>MLGLKTSIIGRRVIYFQEITSTNEFAKTSYLEEGTVIVADKQTMGHGALNRKWESPEGGLWLSIVLSPKVPQKDLPKIVFLGAVGVVETLKEFSIDGRIKWPNDVLVNYKAIAGVLVEGKGDKIVLGIGLNVNNKVPNGATSMKLELGSEVPLLSVFRSLITNLDRLYLNFLKNPMDILNLVRDNMILGVRVKILGDGSFEGIAEDIDDFGRLIIRLDSGEVKKVIYGDVSLRFL[2x];>[2x]MVVSENVVSAPMPGKVLRVLVRV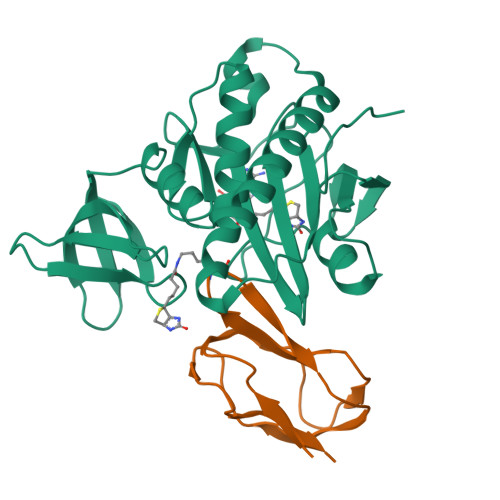GDRVRVGQGLLVLEAMKMENEIPSPRDGVVKRILVKEGEAVDTGQPLIELG N-(carboxycarbonyl)-S-(naphthalen-2-ylmethyl)-L-cysteine 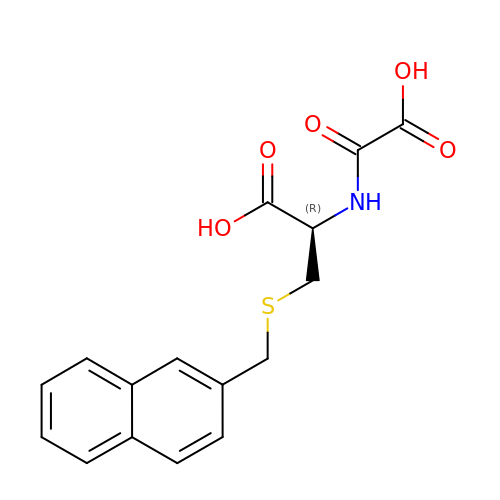| C16 H15 N O5 S | TUTBXYUXRIILSH-ZDUSSCGKSA-N>[4x]MNFRGHALPGTFFFIIGLWWCTKSILKYICKKQKRTCYLGSKTLFYRLEILEGITIVGMALTGMAGEQFIP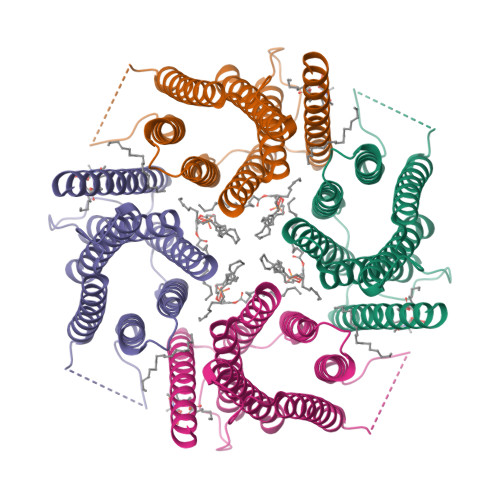GGPHLMLYDYKQGHWNQLLGWHHFTMYFFFGLLGVADILCFTISSLPVSLTKLMLSNALFVEAFIFYNHTHGREMLDIFVHQLLVLVVFLTGLVAFLEFLVRNNVLLELLRSSLILLQGSWFFQIGFVLYPPSGGPAWDLMDHENILFLTICFCWHYAVTIVIVGMNYAFITWLVKSRLKRLCSSEVGLLKNAEREQESEEEMAENLYFQ N-[(3-{4-amino-5-[3-(benzyloxy)phenyl]-7H-pyrrolo[2,3-d]pyrimidin-7-yl}cyclobutyl)methyl]acetamide | C26 H27 N5 O2 | 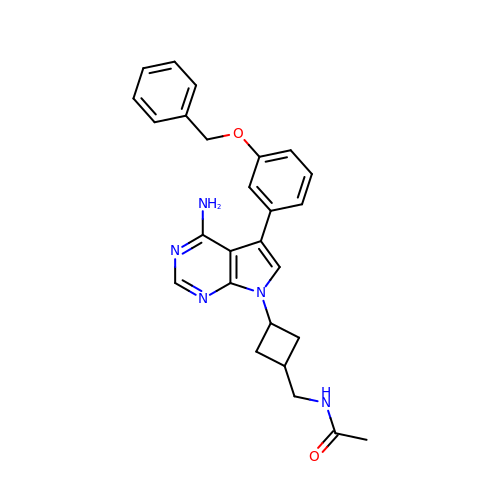BUCAFRXFNHCHRU-UHFFFAOYSA-N The housekeeping enzyme glucose 6-phosphate dehydrogenase (G6PD) (EC 1.1.1.49) is the first and rate-limiting enzyme of the PPP. It catalyzes the oxidation of glucose 6-phosphate (G6P) originating from glycolysis to 6-phospho-D-glucono-1,5-lactone (6PL), whereby the cofactor NADP+ is reduced to NADPH. In the present study, we describe the crystal structures of Leishmania donovani G6PD (LdG6PD), both native and complexed with one or both substrates. The LdG6PD monomer contains three domains: an N-domain (Q5-K49), the NADP+ binding “Rossmann-like” domain (residues D50-I248), and a β + α domain (residues D249-K552).

The crystals of the apoenzyme obeyed P121 symmetry with four monomers in the asymmetric unit (AU) and diffracted to 2.8 Å. The apo form crystallizes in space group P121 with two dimers (AB and CD) in the AU. Via P121 symmetry operation, a tetramer can be formed from each dimer (ABA’B’ or CDC’D’). Comparing the apo structure with the structures complexed with G6P, NADP(H) or both substrates reveals a rotation of the N-domain by about 45° upon ligand binding. In the apo structure, the N-domain of subunit A (NA) interacts with the flexible loop (T471-D482) of both subunits. Within subunit A, the helical residues A26A-E30A (α1) interact with loop residues Y472A-Y476A. Residues E30A-K32A are bound to the β-strand S442A-A444A (β13). Furthermore, the R31A side chain interacts with E467A and D469A (β14). Additionally, NA (apo structure) interacts with not only subunit A but also B; the N-terminus of helix α2A (Q38A) is bonded to the flexible loop residues T471B and H473B. Linking P1 to subunit B, results in no dimeric interactions between NB and subunit A, but in all our structures there are multiple contacts with the “Rossmann-like” domain of subunit B. In the apo form, α1B (A12B-Q27B) interacts via van der Waals forces with the helical residues D117B-W121B (α4B) and E135B-E141B (α5B).

>MSEEQSHADQDAYVADVDGILDVLRAQVLERKPDDIFQFISKSALSLQKDRGAESCDRINCKVKDEQKSRALTIIVFGASGDLAKKKTFPALFDLYCGGLLPPEVNIIGYARTKVDDVEKWKHETLMKYFSNLSERGCHAEDFLKHISYFCGAYDSVDDFKRLDAVIREKENAFKGPEKGGNRLFYLALPPSVFASVCESIHKGAMPQEVGGWVRVIIEKPFGRDTKSSAELSQALEPFFDESQLYRIDHYLGKEMVQNIITTRFANRIFSAVWNASNIACVQITFKETIGTEGRGGYFDNIGIIRDVMQNHLTQILALLAMEKPRSLDAECIRDEKVSVLKCIEPITKENCVLGQYTASADGSIPGYLEDVTVPEGSTCPTFAVMRLNINNDRWAGVPFILKAGKAVEQKYVAIRIQFRDEVHPYGEATQRNELVIRAQPSEAMYVKITTKVPGLSGDLRQTHQTELDLTYHTRYDVRLPDAYESLINDALLGNSTNFVRKDELDVAWRIFTPLLHQIDSGEIKPIPYQAGTRGPKEADEFIANNGFKHQKGYHWLPSNKL[4x]> AQGPVHLNYRQKGVIDVFLHAWKGYRKFAWGHDELKPVSRSFSEWFGLGLTLIDALDTMWILGLRKEFEEARKWVSKKLHFEKDVDVNLF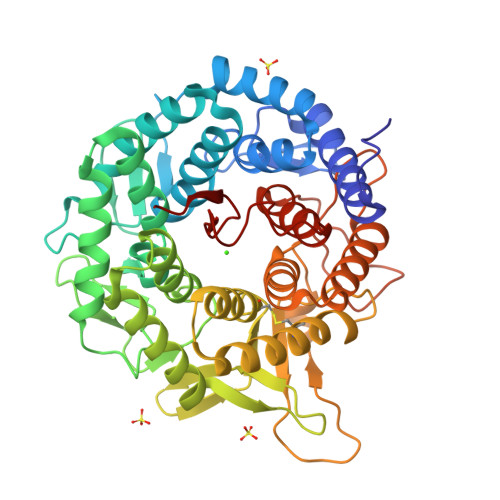ESTIRILGGLLSAYHLSGDSLFLRKAEDFGNRLMPAFRTPSKIPYSDVNIGTGVAHPPRWTSDSTVAEVTSIQLEFRELSRLTGDKKFQEAVEKVTQHIHGLSGKKDGLVPMFINTHSGLFTHLGVFTLGARADSYYEYLLKQWIQGGKQETQLLEDYVEAIEGVRTHLLRHSEPSKLTFVGELAHGRFSAKMDHLVCFLPGTLALGVYHGLPASHMELAQELMETCYQMNRQMETGLSPEIVHFNLYPQPGRRDVEVKPADRHNLLRPETVESLFYLYRVTGDRKYQDWGWEILQSFSRFTRVPSGGYSSINNVQDPQKPEPRDKMESFFLGETLKYLFLLFSDDPNLLSLDAYVFNTEAHPLPIWT>[2x]MSRLDKSKVI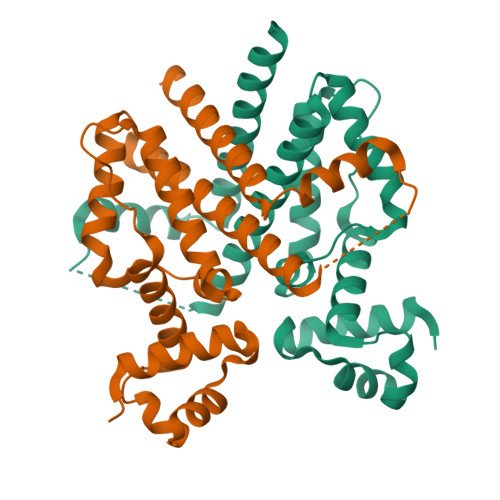NSALELLNEVGIEGLTTRKLAQKLGVEQPTLYWHVKNKRALLDALAVEILARHKDYSLPAAGESWQSFLRNNAMSFRRALLRYRDGAKVHLGTRPDEKQYDTVETQLRFMTENGFSLRDGLYAILAVIHFTLGAVLEQQEHTAALTDRPAAPDENLPPLLREALQIMDSDDGEQAFLHGLESLIRGFEVQLTALLQIV> DDYSVVEEHGQLSISNGELVNERGEQVQLKGMSSHGLQWYGQFVNYESMKWLRDDWGITVFRAAMYTSSGGYIDDPSVKEKVKETVEAAIDLGIYVIIDWHILSDNDPNIYKEEAKDFFD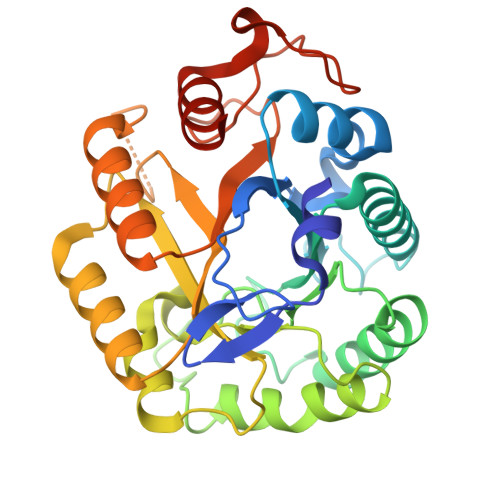EMSELYGDYPNVIYEIANEPNGSDVTWDNQIKPYAEEVIPVIRDNDPNNIVIVGTGTWSQDVHHAADNQLADPNVMYAFHFYAGTHGQNLRDQVDYALDQGAAIFVSEWGTSAATGDGGVFLDEAQVWIDFMDERNLSWANWSLTHKDESSAALMPGANPTGGWTEAELSPSGTFVREKIRESASIPP[(1R)-1-{[6-(4-methylphenyl)thieno[2,3-d]pyrimidin-4-yl]amino}-2-phenylethyl]phosphonic 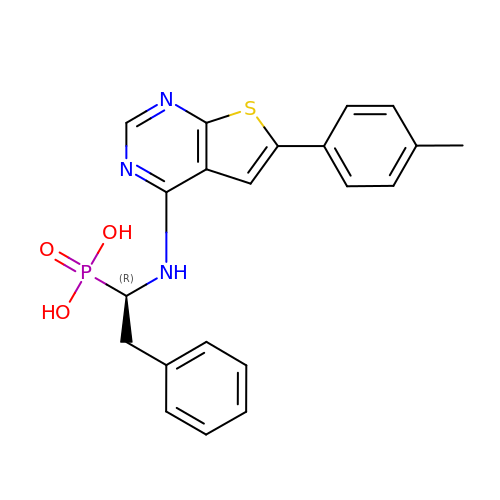acid | C21 H20 N3 O3 P S | UYKRLVOVLULTHW-LJQANCHMSA-N Ubiquitin-specific proteases (USPs)5 are key players in the regulation of important cellular signaling pathways through catalyzing the deconjugation reaction of ubiquitin from substrate proteins. The multifunctional protease USP15 regulates several important pathways in health and disease, including TGF-β, IGF-I, innate immune signaling, mRNA processing, and mitophagy. USP15, USP4, and USP11 share the same overall domain structure, including an N-terminal domain present in USPs (DUSP) and ubiquitin-like (UBL) domain followed by a protease domain that harbors a ∼300-amino acid insertion predicted to contain a second UBL domain. The USP15 catalytic core displays the characteristic USP protease domain fold, including a finger, palm, and thumb region.

Furthermore, we determined the structure of a USP15–mitoxantrone complex, a Food and Drug Administration–approved antineoplastic drug, which has multiple cellular targets, including USP11 (25), that shows a novel binding mode for a USP ligand. We determined that USP15 is weakly inhibited by mitoxantrone with an IC50 value of 33 ± 11 μm. Co-crystallization trials in the presence of excess mitoxantrone yielded crystals of intense blue color that diffracted to 2.1 Å resolution (data collection and refinement statistics are shown in Table 1). After molecular replacement, an additional planar shape of electron density was visible in the vicinity of the BL2 region near the catalytic histidine that corresponded to the anthracenedione structure of mitoxantrone. The catalytic triad in this different crystal form is also misaligned in both USP15 copies present in the asymmetric unit in a similar configuration to the USP15-free enzyme structure. This USP15–mitoxantrone complex structure revealed predominantly hydrophobic interactions between mitoxantrone and USP15 residues Tyr855, Gly856, Gly860, His862, which are located in the BL2 region. In addition, one of mitoxantrone's side arms contacts the CC loop Asn264, although the density is weaker compared with the mitoxantrone anthracenedione core. There are no interactions of mitoxantrone with other neighboring USP15 molecules in the crystal lattice. This binding site coincides with the S1′ region of USP15, suggesting a rationale for the inhibition observed. In this position, mitoxantrone is expected to compete with substrate interactions, as indicated by modeling a diubiquitin molecule into the binding site based on a superposition with a USP30 C77A Lys6-linked diubiquitin structure, the closest available USP structure in complex with a substrate. Superposition of the USP15-free and mitoxantrone-bound structures revealed that the BL2 becomes ordered, but no other major conformational changes are observed upon mitoxantrone binding.

>MEQPGLCGLSNLGNTCFMNSAIQCLSNTPPLTEYFLNDKYQEELNFDNPLGMRGEIAKSYAELIKQMWSGKFSYVTPRAFKTQVGRFAPQFSGYQQQDCQELLAFLLDGLHEDLNRIRKKPYIQLKDADGRPDKVVAEEAWENHLKRNDSIIVDIFHGLFKSTLVCPECAKISVTFDPFCYLTLPLASTSKVKLKDCIELFTTKEKLGAEDPWYCPNCKEHQQATKKLDLWSLPPVLVVHLKRFSYSRYMRDKLDTLVDFPINDLDMSEFLINPNAGPCRYNLIAVSNHYGGMGGGHYTAFAKNKDDGKWYYFDDSSVSTASEDQIVSKAAYVLFYQRQDTFSGTGFFPLDRETAAALEHHHHHH[2x]>MGSSHHHHHHSSGLVP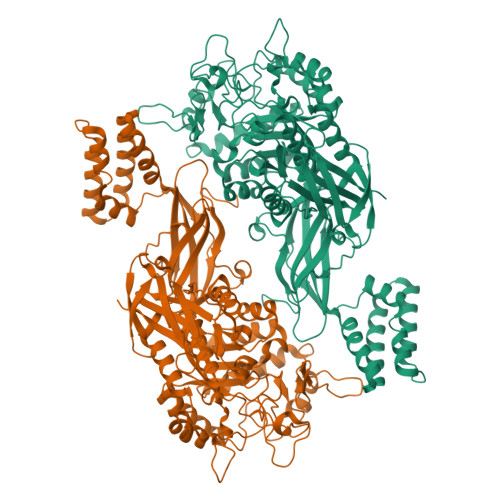RGSHMPATHHSSATSAERPTVVGRIPVLDVRPVVQRGRRPAKAVTGESFEVSATVFREGHDAVGANVVLRDPRGRPGPWTPMRELAPGTDRWGATVTAGETGTWSYTVEAWGDPVTTWRHHARIKIPAGLDTDLVLEEGARLYERAAADVPGREDRRELLAAVDALRDESRPAASRLAAALTPQVDAVLARHPLRDLVTSSDPLPLLVERERALYGAWYEFFPRSEGTPHTPHGTFRTAARRLPAIAAMGFDVVYLPPIHPIGTTHRKGRNNTLSATGDDVGVPWAIGSPEGGHDSIHPALGTLDDFDHFVTEAGKLGLEIALDFALQCSPDHPWVHKHPEWFHHRPDGTIAHAENPPKKYQDIYPIAFDADPDGLATETVRILRHWMDHGVRIFRVDNPHTKPVAFWERVIADINGTDPDVIFLAEAFTRPAMMATLAQIGFQQSYTYFTWRNTKQELTEYLTELSGEAASYMRPNFFANTPDILHAYLQHGGRPAFEVRAVLAATLSPTWGIYSGYELCENTPLREGSEEYLDSEKYQLKPRDWTRAAREGTTIAPLVTRLNTIRRENPALRQLRDLHFHPTDKEEVIAYSKRQGSNTVLVVVNLDPRHTQEATVSLDMPQLGLDWHESVPVRDELTGETYHWGRANYVRLEPGRTPAHVCTVLRPSHPQIGGSHTT[4x]>[2x]MASKGNVDLVFLFDGSMSLQPDEFQKILDFMKDVMKKLSNTSYQFAAVQFSTSYKTEFDFSDYVKWKDPDALLKHVKHM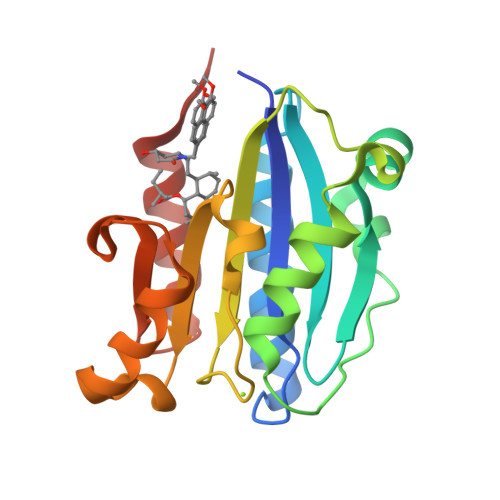LLLTNTFGAINYVATEVFREELGARPDATKVLIIITDGEATDSGNIDAAKDIIRYIIGIGKHFQTKESQETLHKFASKPASEFVKILDTFEKLKDLFTELQKKIYVIEG>TETTSFSITKFSPDQQNLIFQGDGYTTKGKLTLTKAVKSTVGRALYSTPIHIWDRDTGNVANFVTSFTFVIDAPSSYNVADGFTFFIAPVDTKPQTGGGYLGVFNSKEYDKTSQTVAVEFDTFYNAAWDPSNKERHIGIDVNSIKSVNTKSWNLQNGERANVVI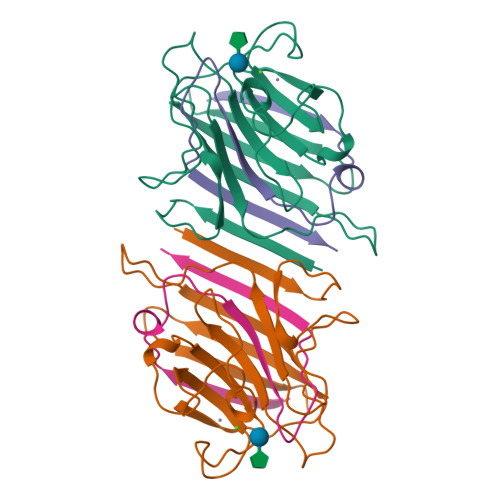AFNAATNVLTVTLTYPN[2x];>VTSYTLNEVVPLKDVVPEWVRIGFSATTGAEFAAHEVHSWSFHSQLGHTSKS[2x]> MQLTPTFYDNSCPNVSNIVRDTIVNELRSDPRIAASILRLHFHDCFVNGCDASILLDNTTSFRTEKDAFGNANSARGFPV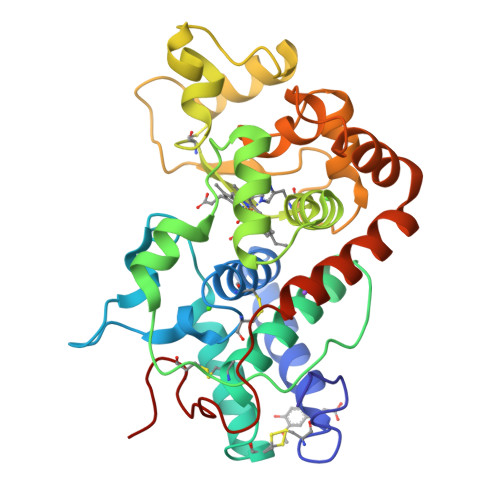IDRMKAAVESACPRTVSCADLLTIAAQQSVTLAGGPSWRVPLGRRDSLQAFLDLANANLPAPFFTLPQLKDSFRNVGLNRSSDLVALSGGHTFGKNQCRFIMDRLYNFSNTGLPDPTLNTTYLQTLRGLCPLNGNLSALVDMDLRTPTIFDNKYYVNLEEQKGLIQSDQELFSSPNATDTIPLVRSFANSTQTFFNAFVEAMDRMGNITPLTGTQGQIRLNCRVVNSNS S2P intramembrane metalloproteases regulate diverse signaling pathways across all three domains of life. Here we determine the cryo-EM structure of the S2P family intramembrane metalloprotease SpoIVFB from Bacillus subtilis bound to its native substrate Pro-σK. The structure and accompanying biochemical data demonstrate that SpoIVFB positions Pro-σK at the enzyme active site through a β-sheet augmentation mechanism, and reveal key interactions between Pro-σK and the interdomain linker connecting SpoIVFB transmembrane and CBS domains. Finally, the zinc-metalloprotease activity of SpoIVFB results in cleavage of the N-terminal pro-sequence of Pro-σK within the interior of the lipid membrane, allowing the mature σK to diffuse from the outer forespore membrane into the mother cell cytoplasm, bind to RNA polymerase core subunits, and initiate transcription of genes involved in the final stages of B. subtilis spore maturation (step 3).

Thus, although WT SpoIVFB appears to display robust enzymatic activity in E. coli, this activity is lost after detergent solubilization and purification of WT SpoIVFB and Pro-σK. To further investigate the overall architecture of detergent-solubilized SpoIVFB and Pro-σK preparations, we pursued cryo-EM reconstructions of both WT and E44Q SpoIVFB co-purified with Pro-σK. In total, the physical interaction between monomers in the WT SpoIVFB:Pro-σK tetramer is quite limited (~488Å2 for interface 1, ~510Å2 for interface 2), which likely makes for fragile interactions between SpoIVFB:Pro-σK monomers that are largely mediated by lipid/detergent. As elaborated on below and in the discussion, we believe that the oligomeric arrangement of SpoIVFB:Pro-σK monomers in the tetramer is likely an artifact of detergent solubilization, rather than a representation of an oligomeric state that is sampled in vivo. Aside from the difference in oligomeric state, which we believe arises simply from variations between protein preparations and fragile monomer interfaces, the final structures of WT and E44Q SpoIVFB:Pro-σK monomers are virtually superimposable (RMSD ~ 0.5 Å). For this reason, we refer to WT SpoIVFB:Pro-σK in the following presentation of results due to the slightly higher overall resolution obtained for this complex. While the orientation of zinc-coordinating residues H43, H47, and D137 of SpoIVFB are conserved with those of mjS2P, the cryo-EM map of WT SpoIVFB:Pro-σK does not show any appreciable density for an ion being coordinated by these residues. This lack of density was consistent in the cryo-EM maps of both WT and E44Q SpoIVFB:Pro-σK, demonstrating that SpoIVFB:Pro-σK complexes fail to co-purify with the Zn2+ ion that is essential for supporting Pro-σK cleavage. Thus, the cryo-EM maps provide an explanation for why WT SpoIVFB consistently co-purifies with full-length unprocessed Pro-σK despite displaying robust proteolytic activity in E. coli.

>[4x]MNKWLDLILKIHVHPFLWIIAALGLLTGHMKALLCLLLIVLIHELGHAALAVFFSWRIKRVFLLPFGGTVEVEEHGNRPLKEEFAVIIAGPLQHIWLQFAAWMLAEVSVIHQHTFELFTFYNLSILFVNLLPIWPLDGGKLLFLLFSKQLPFQKAHRLNLKTSLCFCLLLGCWVLFVIPLQISAWVLFVFLAVSLFEEYRQRHYIHVRFLLERYYGKNRELEKLLPLTVKAEDKVYHVMAEFKRGCKHPIIIEKSGQKLSQLDENEVLHAYFADKRTNSSMEELLLPYKLDYKDDDDKDYKDDDDKLEHHHHHH;>MVTGVFAALGFVVKELVFLVSYVKNNAFPQPLSSSEEKKYLELMAKGDEHARNMLIEHNLRLVAHIVKKFENTGEDAEDLISIGTIGLIKGIESYSAGKGTKLATYAARCIENEILMHLRALKKTKKGSHHHHHH[4x]> GAMGNNTEAISELQSSPIKLGKIKVLQKTEKIVSTQNLQNLQQSQFFKNEKEKIIKKIAQEFDENEKLINKIGPNIEMFAQTINTDIQKIEPNDQFGI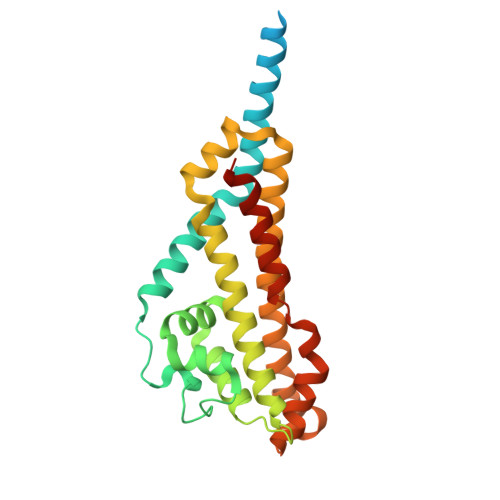NKTLFTEKKDNNIDFMLKDNRLRRLFYSSLNYDENKIKKLATILAQTSSSNDYHYTLIGLIFWTGFKIQEAFESAVNILTKDEQKRLIFNFRTKTVKEIQENFEKLMQERNSWIKIVDNIIGEYDKNTGGCKADGKILGEVIRVGYEHELDSNKSMQILNNIETPLKTCCDHIHY>MGSSHHHHHHSSGLVPRGSHMTAPGHTSVQTPIAGLVELALSDPSLQDVIRRAADRPADLALVGPASARVLVAAALAQNGPLLVVAATGREADELTAELRGVFGDSVALFPSWETLPHERLSPGVETVGARLMLLRRLARPDDETLGAPLRVVVTTTRSLLQPMAPDLVDIEPVTLSVGAEMEFEDVVARLVDLSYTRVDMVGKRGEFAVRGGILDVFPPTAEHPVRVEFWGDEISEMRAFAIADQRSIPEVPVQTVVAVPCRELLMTDDVRERAAALAAEHPTTENTVPGTVPDMLAKLAEGIPVDGMEALLPLLHPIEPTTLTRHLPEGAPVLVCDPEKVRTRAADLIKTGREFLEASWSTAAVGGDAPIDLEALGASGFVTFEEAREAAREGGHPWWTLSQLSDESAVELDIRSAPSARGSQHNLEEIFAMLRAHVATGGYAAVVTPGIGTAHRVVEQLGEADTAATILEPGTAPKAGVVGVLKGPLCSGVVLPGANLVIITETDLTGNRVTANEGRKLAAKRRNVVDPLALTAGDLVVHDQHGIGKFVEMTERVVGGARREYLVLEYASSKRGGGTDKLYVPMDSLDQLSRYVGGEAPSLSRLGGSDWANTKTKARRAVREIASELVALYAKRQSAPGHAFGPDTPWQAEMEDAFGFTETIDQLTAIQEVKSDMEKPVPMDRVICGDVGYGKTEIAVRAAFKAVQDGKQVAVLVPTTLLADQHLQTFTNRMAGFPVTVKGLSRFTDPAESRAVIEGLKDGSVDVVIGTHRLLQTGVTWKDLGLIIVDEEQRFGVEHKEHIKSMRTHVDVLTMSATPIPRTLEMSLAGIREMSTILTPPEERYPVLTYVGPHDDKQVAAALRRELLRDGQAFYIHNRVRTIDEAAARVRQLVPEARVVVAHGQMNEETLEKTVEGFWNREYDILVCTTIVETGLDISNANTLIVERADTFGLSQLHQLRGRVGRSRERGYAYFLYPPNKPLTETAYDRLATIAQNNELGAGMAVAMKDLEIRGAGNVLGAEQSGHVAGVGFDLYVRLVGEAVEAYRAAADGKTVATPQEQKDVRIDLPVDAHLPPEYIGSDRLRLEAYRRLAAAADDDAVASVVDELIDRYGPLPEPAQRLVAVARLRLLCREFGITEIGAVSASTVRLSPMVLPDSAQLRLKRMYPGGHYRATTSTVQVPLPRAGEGVGAPRIRDLELVQWVAGLVLVLNGKGQGDVD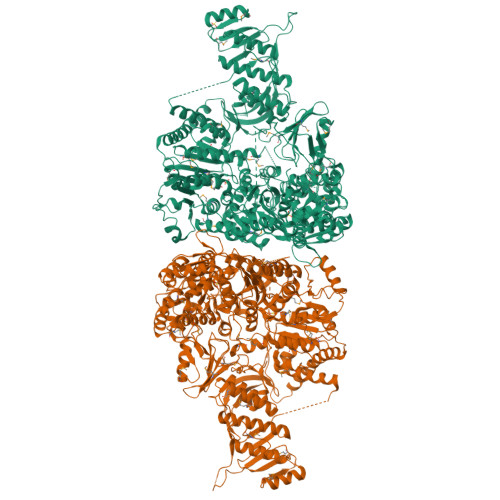MSKFSNPAGEAKR[2x]(2R,3S,4R)-3-(2'-fluoro[1,1'-biphenyl]-4-yl)-4-(hydroxymethyl)azetidine-2-carbonitrile | C17 H15 F N2 O | 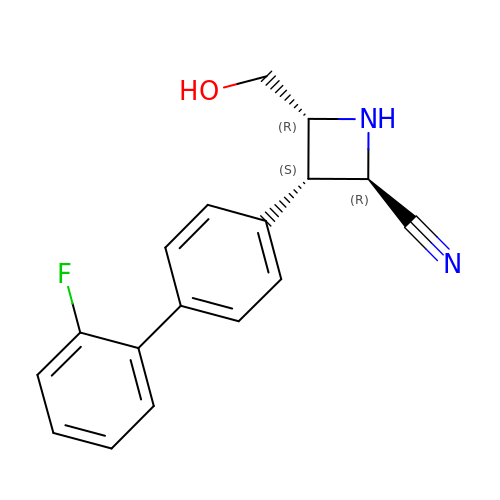RECLLIAWOQFAMC-ULQDDVLXSA-N>[2x]MSFPKGFLWGAATASYQIEGAWNEDGKGESIWDRFTHQKGNILYGHNGDV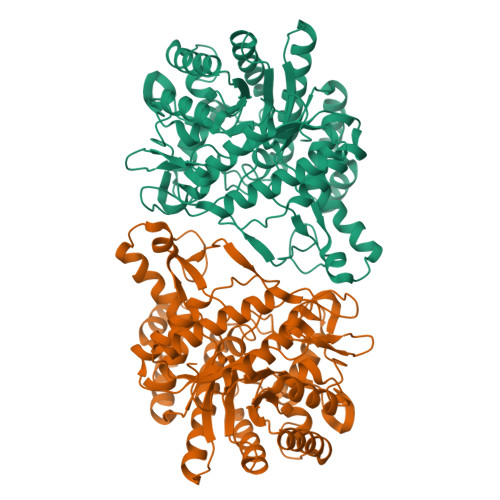ACDHYHRHEEDVSLMKELGIKAYRFSTAWARIFPDGFGNINQKGLEFYDKLINELVENGIEPVVTLYHWDLPQKLQDIGGWANPEIVNYYFEYAMLIINRYKDKVKKWITFNEPYCIAFLGHWHGIHAPGIKNFKVAMDVVHNIMLSHFKVVKAVKENNIDVEIGITLNLTPVYLQTERLGYKVSEIEREMVNLSSQLDNELFLDPVLKGSYPQKLLDYLVQKDLLDSQKVNNMQQEVKENFIFPDFLGINYYTRSVRLYDENSGWIFPIRWEHPAGEYTEMGWEVFPQGLFDLLIWIKESYPQIPIYITENGAAYNDKVEDGRVHDQKRVEYLKQHFEAARKAIKNGVDLRGYFVWSLIDNFEWAMGYTKRFGIIYVDYETQKRIKKDSFYFYQQYIKENSLE>[2x]TETTSFSITKFSPDQQNLIFQGDGYTTKGKLTLTKAVKSTVGRALYSTPIHIWDRDTGNV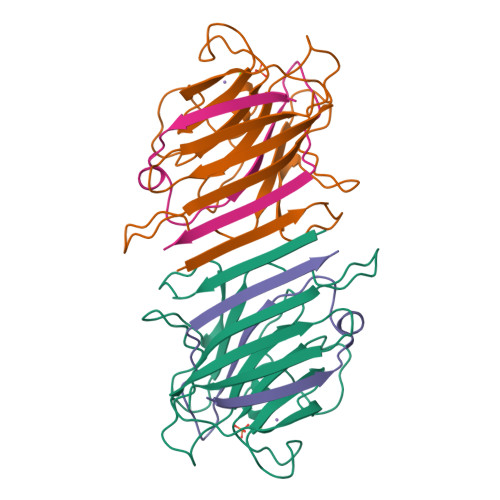ANFVTSFTFVIDAPSSYNVADGFTFFIAPVDTKPQTGGGYLGVFNSKEYDKTSQTVAVEFDTFYNAAWDPSNKERHIGIDVNSIKSVNTKSWNLQNGERANVVIAFNAATNVLTVTLTYPN;>VTSYTLNEVVPLKDVVPEWVRIGFSATTGAEFAAQEVHSWSFNSQLGHTSKS[2x]> GPLGSEKIEKDNAFAFDLLQTTRKHVTEANVFISPLSVSMALNMTLNGAAGVTADEMKTALRETGYTMEDINEYSHSLREALLKVDPSTTIGMANSIWYKQGELVKEPFILANRTHYDAEVKAVDFSSPATLPAINGWCAQKTNDKITKILDYIPGNAFMYLINAVYFKGIWVTQFKKSDTKRAPFRKADGTTQEVNMMAQKSTFGYTTDECCQYLEMDYGNKAFSMIVMLPNEGQTTRDVIEQLDNKHWSMIIKGIRPTQVSLRMPRFKTECKYGLEKKILPEMGMNVPFTETADFPGITDAAIFISRVIHKTFVQVD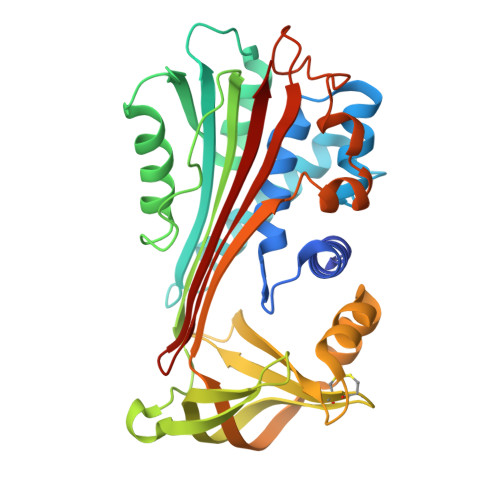EEGTEAAAVTAVEMVK>[4x]MEGGSITPGEDKPEIQSPIPPNQIFILSGQSNMAGRGGVFKDHHNNRWVWDKILPPECAPNSSILRLSADLRWEEAHEPLHVDIDTGK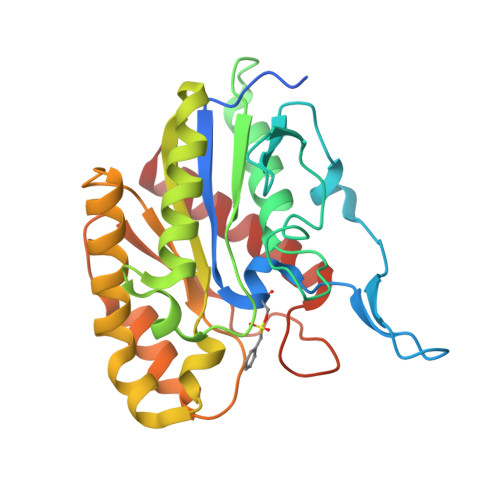VCGVGPGMAFANAVKNRLETDSAVIGLVPCASGGTAIKEWERGSHLYERMVKRTEESRKCGGEIKAVLWYQGESDVLDIHDAESYGNNMDRLIKNLRHDLNLPSLPIIQVAIASGGGYIDKVREAQLGLKLSNVVCVDAKGLPLKSDNLHLTTEAQVQLGLSLAQAYLSNFC> VEGRFQLVAPYEPQGDQPQAIAKLVDGLRRGVKHQTLLGATGTGKTFTISNVIAQVNKPTLVIAHNKTLAGQLYSELKEFFPHNAVEYFVSYYDYYQPEAYVPQTDTYIEKDAKINDEIDKLRHSATSALFERRDVIIVASVSCIYGLGSPEEYRELVVSLRVGMEIERNALLRRLVDIQYDRNDIDFRGTFRVRGDVVEIFPASRDEHCIRVEFFGDEIERIREVDALTGKVLGEREHVAIFPASHFVTREEKMRLAIQNIEQELEERLAELRAQGKLLEAQRLEQRTRYDLEMMREMGFCSGIENYSRHLALRPPGSTPYTLLDYFPDDFLIIVDESHVTLPQLRGMYNGDRARKQVLVDHGFRLPSALDNRPLTFEEFEQKINQIIYVSATPGPYELEHSPGVVEQIIRPTGLLDPTIDVRPTKGQIDDLIGEIRERVERNERTLVTTLTKKMAEDLTDYLKEAGIKVAYLHSEIKTLERIE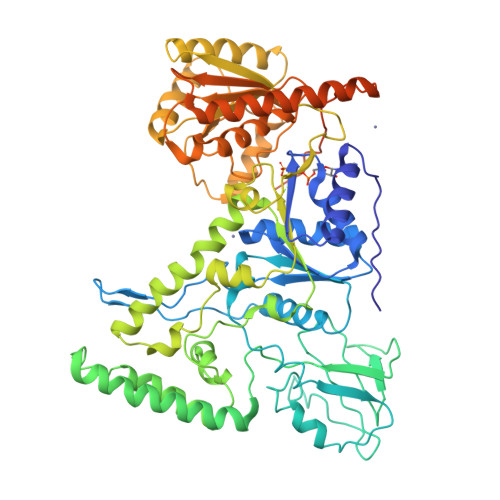IIRDLRLGKYDVLVGINLLREGLDIPEVSLVAILDADKEGFLRSERSLIQTIGRAARNANGHVIMYADTITKSMEIAIQETKRRRAIQEEYNRKHGIVPRTVKKEIRDVIRATYAAEETEMYEAKPAAAMTKQEREELIRTLEAEMKEAAKALDFERAAQLRDIIFELKAEG>EVYALEESRDVYLSDLDWLNATHGDDTKSKIVQKNHPFTPGNNNQSTKISLKMEDGSISEFEKGLGTIAGSPSTITYDISGAGVTKFFSYLGIDRSANPINEQYAKVDKIEVVVDGKVIYSTINQFPNGLTYETPAIKVDLNIPENAKRL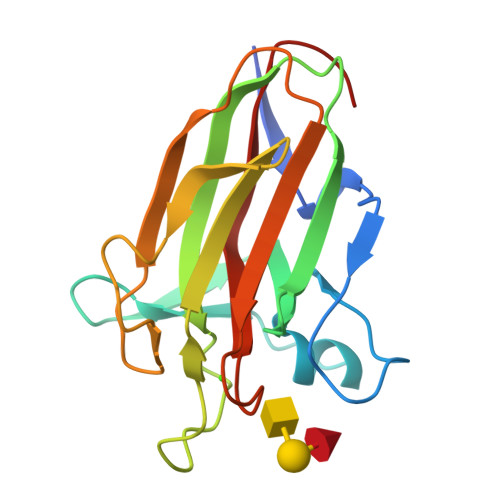QLKSYAGEKTWGDEVVYADAKFTAKGDFVN[2x]> STAAVTGQTGLTITYPASATESAAIQGTFGNSAAIKIKNQTLTWTRTPEGAWSC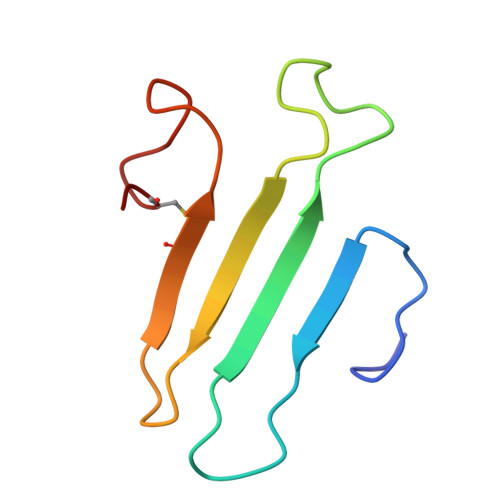ATTVEAKFKPAGCAS>MNFGAFSINPAMMAAAQAALQSSWGMMGMLASQQNQSGPSGNNQNQGNMQ[10x];>GMLAS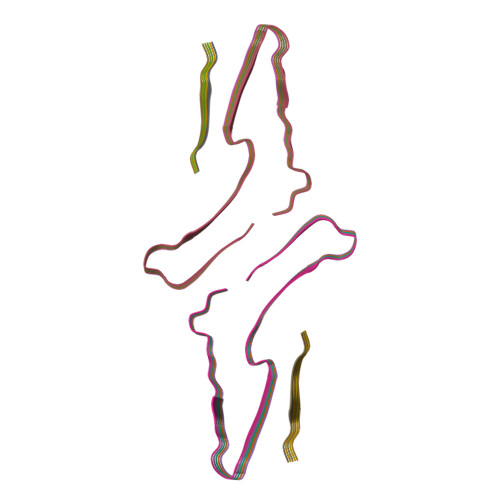QQNQS[10x]>MGSSHHHHHHSGESYPQRQ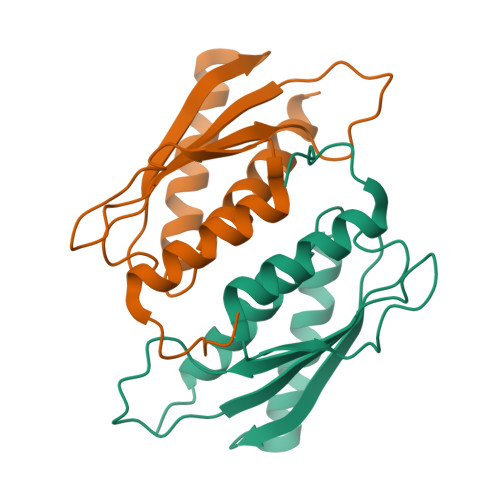DHELQALEAIYGADFQDLRPDACGPVKEPPEINLVLYPQGLTGEEVYVKVDLRVKCPPTYPDVVPEIELKNAKGLSNESVNLLKSRLEELAKKHCGEVMIFELAYHVQSFLSEHNK[6x]> STKEKPKPTPDYLMQLMNDKKLMSSLPNFCGIFNHLERLLDEEISRVRKDMYNDTLNGSTEKRSAELPDAVGPIVQLQEKLYVPVKEYPDFNFVGRILGPRGLTAKQLEAETGCKIMVRGKGSMRDKKKEEQNRGKPNWEHLNEDLHVLITVEDAQ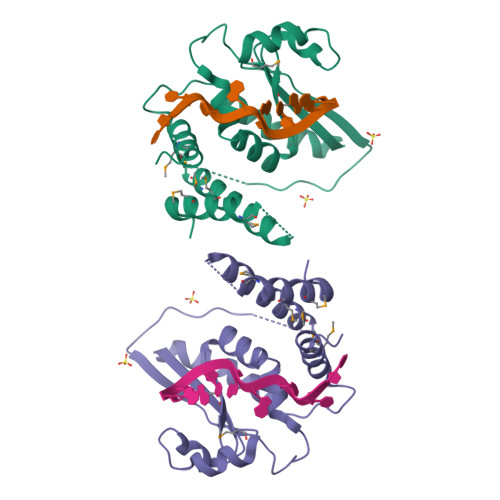NRAEIKLKRAVEEVKKLLVPAAEGEDSLKKMQLMELAILNGTYRDANIKSPAL>AMDPEFETGEVVDCHLSDMLQQLHSVNASKPSERGLVRQEEAEDPACIPIFWVSKWVDYSDKYGLGYQLCDN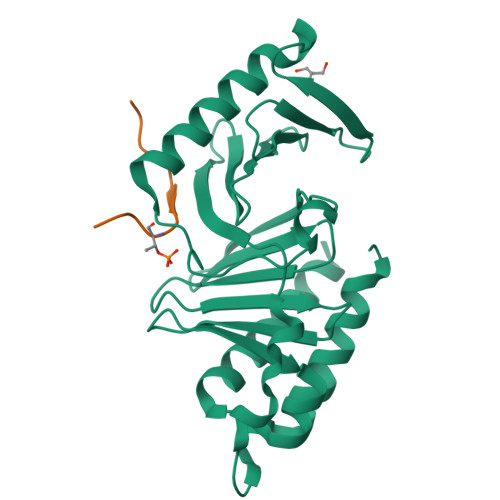SVGVLFNDSTRLILYNDGDSLQYIERDGTESYLTVSSHPNSLMKKITLLKYFRNYMSEHLLKAGANITPREGDELARLPYLRTWFRTRSAIILHLSNGSVQINFFQDHTKLILCPLMAAVTYIDEKRDFRTYRLSLLEEYGCCKELASRLRYARTMVDKLLSSRSASNRLKAS[2x];>WSSSLATPPTLSSTVLI[2x]>[2x]SCPDACCPHGSSGLRCTRDGALDSLHHLPGAENLTELYIENQQHLQHLELRDLRGLGELRNLTIVKSGLRFVAPDAFHFTPRLSRLNLSFNALESLSWKTVQGLSLQELVLSGNPLHCSCALRWLQRWEEEGLGGVPEQKLQCHGQGPLAHMPNASCGVPTLKVQVPNASVDVGDDVLLRCQVEGRGLEQAGWILTELEQSATVMKSGGLPSLGLTLANVTSDLNRKNLTCWAENDVGRAEVSVQVNVSFPASVQLHTAVEMHHWCIPFSVDGQPAPSLRWLFNGSVLNETSFIFTEFLEPAANETVRHGCLRLNQPTHVNNGNYTLLAANPFGQASASIMAAFMDNPAAAHHHHHHHH;>[2x]MSHHHHHHHHSENLYFQSGGGRDEIKERIFKAVVRAIVTGNPEQLKEAKKLLEKLKKLGRLDQDAKKFEKAIRQVEKRLRS

The design of proteins that bind to a specific site on the surface of a target protein using no information other than the three-dimensional structure of the target remains a challenge. Here we describe a general solution to this problem that starts with a broad exploration of the vast space of possible binding modes to a selected region of a protein surface, and then intensifies the search in the vicinity of the most promising binding modes. We demonstrate the broad applicability of this approach through the de novo design of binding proteins to 12 diverse protein targets with different shapes and surface properties. Biophysical characterization shows that the binders, which are all smaller than 65 amino acids, are hyperstable and, following experimental optimization, bind their targets with nanomolar to picomolar affinities.

We succeeded in solving crystal structures of five of the binder–target complexes, and all five closely match the corresponding computational design models.>SNEKIRSQSVLNTLETFFIKENHYDMQREESSIVNACLRYLGYSKSMCHEKMPIFMDIAFIEYCFNLSLDPSSFQNLPITQTQPDSQQILWEYSLISNALERLENIELERQNCMREDGLSKYTNSLLLNKETLNNEALKLYSCAKAGICRWMAFHFLEQEPIDHINFTKFLQDWGSHNEKEMEALQRLSKHKIRKRLIYVSQHKKKMPWSKFNSVLSRYIQCTKLQLEVFCDYDFKQREIVKMLTSNIN[4x];>SEACEMCRLGLPHGSFFELL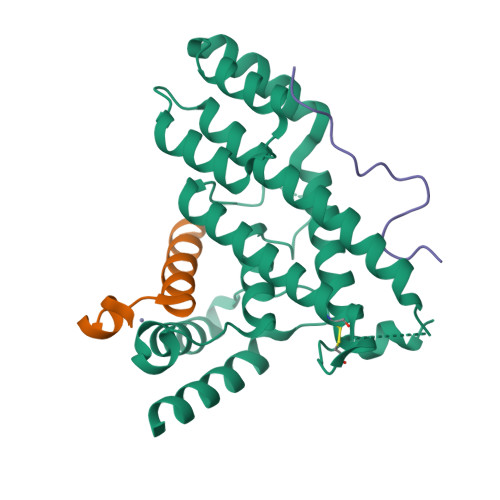RDWKKIEEFRNKS[4x];>SDNIFVKPGEDLEIPLLSDYSDSENISEKS[4x]> MIERGKFRSLTLVNWNGFFARTFDLDELVTTLSGGNGAGKSTTMAAFVTALIPDLTLLHFRNTTEAGATSGSRDKGLHGKLRAGVCYSTLDVINSRHQRVVVGVRLQQVAGRDRKVDIKPFMIQGLPTAIQPTQLLTENVGERQARVLPLNELKDRLDEMEGVQFKQFNSITDYHAQMFDLGVIPKRLRSASDRSKFYRLIEASLYGGISSAITRSLRDYLLPENSGVRKAFQDMEAALRENRITLEAIRVTQSDRDLFKHLITEATSYVSADYMRHANERRTHLDEALALRGELFGSHKQLATEQYRHVEMARELAEQSGASSDLETDHQAASDHLNLVQTAMRQQEKIDRYQVDLEELSYRLEEQTDVVEEAGELQAEYEARTEATEQEVDELKSQLADYQQALDVQQTRAIQYQQALQALERARELCRLPDLSVDNAEEWLETFQAKEQQATEALLALEQKLSVADAAHNQFEQAYQLVKNIVGETSRSEAWQSARELLRDWPSQRHLADRVQPLRMRLSELEQRLNNQQNAERLLSEFCKRQGRQYQAEDLEALQNELEARQEALSLSVNEGGERRMEMRQELEQLKQKIQSLTARAPVWLAAQDTLNQLCEQSGETLASSNDVTEYMQQLLEREREATVERDEVAAQKRELEKQIERLSQPSGAEDSRMIALAERFGGVLLSEIYDDITIDDAPYFSALYGPARHGIVVPDLSLVRPHLETLEDCPEDLYLIEGDPQSFDDSVFNAEEQTNAVLVKSSDRQWRYSRYPELPLFGRAARENRLEALNLERDALAERYATLSFDVQKIQRAHQAFSQFVGKHLSVAFDTDPEAEIRELRQRHTELEREVSRFEDQTQQQRQQYAQAKESLTTLNRLIPQVTLLLDETLIDRVEEVREEMDEAQEAARFLQQHGSALTKLEPMVAVLQSDPQQHEQLQQDYETAKHSQHQAKQQAFALVEIVQRRVHFSYSDSAGMLSENADLNDKLRQRLEHAESDRSRAREQLRQQQAQYSQFNQVLASLKSSYETKQDMLKELLQEMKDIGVQADANAEMRARERRDRLHEA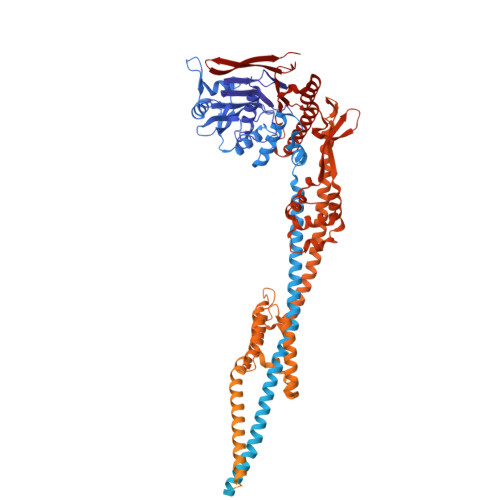LSVNRSRVNQLEKQIAFCEAEMENVQKKLRKLERDYYQIREQVVSAKAGWCAVMRMVKDNGVERRLHRRELAYMEGGALRSMSDKALGALRLAVADNEHLRDALRLSEDPKRPERKVQFFIAVYQHLRERIRQDIIRTDDPVDAIEQMEIELARLTEELTAREQKLAISSKSVANIIRKTIQREQNRIRMLNQGLQAVSFGQVRGVRLNVNVRESHAILLDVLSEQQEQHQDLFNSQRLTFSEAMAKLYQRLNPQVDMGQRLPQTIGEELLDYRNYLELDVEVNRGSDGWLKAESGALSTGEAIGTGMSILVMVVQSWEEESRRLRGKDISPCRLLFLDQAARLDAKSIATLFELCERLQMQLIIAAPENISPEKGTTYKLVRKVFKNHEHVHVVGLRGFGQDAPATQLISDVTA>[2x]MSLIVTVTMNPSIDISYLLDHLKLDTVNRTSQVTKTPGGKGLNVTRVIHDLGGDVIATGVLGGFHGAFIANELKKANIPQAFTSIKEETRDSIAILHEGNQTEILEAGPTVSPEEISNFLENFDQLIKQAEIVTISGSLAKGLPSDFYQELVQKAHA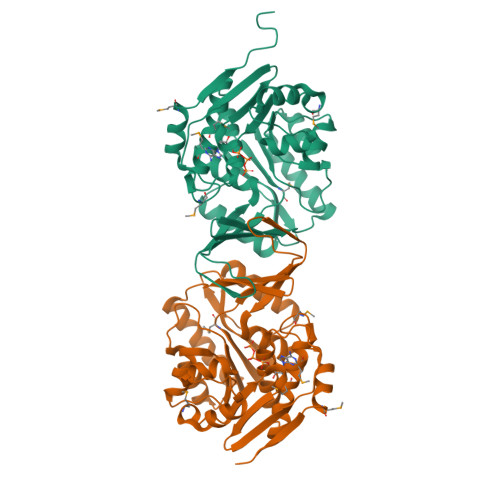QEVKVLLDTSGDSLRQVLQGPWKPYLIKPNLEELEGLLGQDFSENPLAAVQTALTKPMFAGIEWIVISLGKDGAIAKHHDQFYRVKIPTIQAKNPVGSGDATIAGLAYGLAKDAPAAELLKWGMAAGMANAQERMTGHVDVENVKKHLMNIQVVEIAKEGHHHHHH> GAEPYGQKKFIEIAGKRMAYIDEGEGDPIVFQHGNPTSSYLWRNIMPHLEGLGRLIACDLIGMGDSDKLSPSGPDRYSYAEHRDYLFALWEALDLGDNVVLVIHDWGSALGFDWANQHRDRVQGIAYMEAIVTPLEWADWPEEVRDIFQGFRSPAGEEMVLENNIFVERVLPGAILR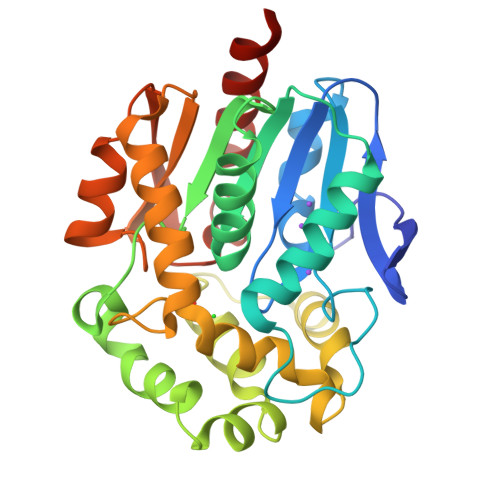QLSDEEMAEYRRPFLNAGEDRRPTLSWPRQIPIDGEPADVVAIVSDYASWLAESDIPKLFINAEPGAIVTGRMRDFCRSWPNQTEITVKGAHFIQEDSPDEIGAAIAEFVRRLRVAAGV(S)-1-(2-cyclopropyl-4-(2-(hydroxymethyl)benzyl)-6-(1,2,3,6-tetrahydropyridin-4-yl)-3,4-dihydroquinoxalin-1(2H)-yl)ethanone | C26 H31 N3 O2 | 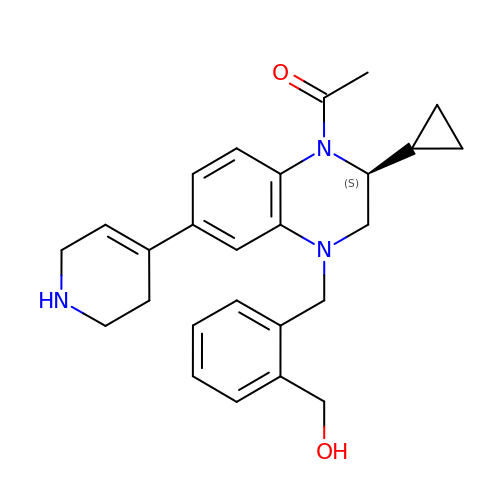ARWMKZDWGIOCEU-AREMUKBSSA-N>MIRVACVGITVMDRIYYVEGLPTESGKYVARNYTEVGGGPAATAAVAAARLGAQVDFIGRVGDDDTGNSLLAELESWGVNTRYTKRYNQAKSSQSAIMVDTKGERIIINYPSPDLLPDAEWLEEIDFSQWDVVLADVRWHDGAKKAFTLA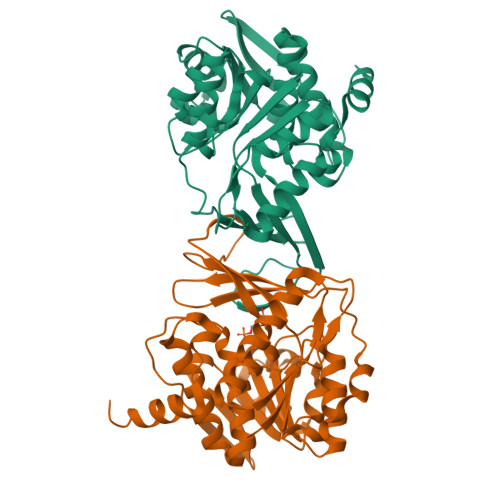RQAGVMTVLDGDITPQDISELVALSDHAAFSEPGLARLTGVKEMASALKQAQTLTNGHVYVTQGSAGCDWLENGGRQHQPAFKVDVVDTTGAGDVFHGALAVALATSGDLAESVRFASGVAALKCTRPGGRAGIPDCDQTRSFLSLFVLEHHHHHH[4x]> MSIKVCIADDNRELVSLLDEYISSQPDMEVIGTAYNGQDCLQMLEEKRPDILLL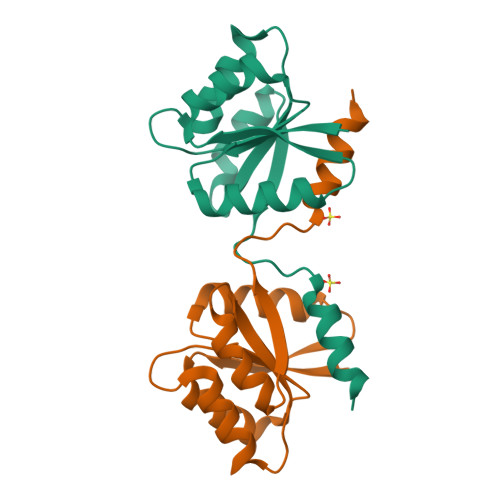DIIMPHLDGLAVLERIRAGFEHQPNVIMLTAFGQEDVTKKAVELGASYFILKPFDMENLAHHIRQVYGKTTPVVRK>MRGSHHHHHHGSMSNFVNLDIFSNYQKYIDNEQEVRENIRIVVREIEHLSKEAQIKLQIIHSDLSQISAACGLARKQVELCAQKYQKLAELVPAGQYYRYSDHWTFITQRLIFIIALVIYLEAGFLVTRETVAEMLGLK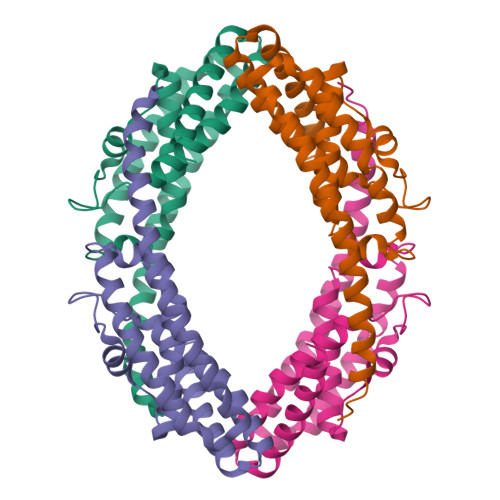ISQSEGFHLDVEDYLLGILQLASELSRFATNSVTMGDYERSLNISHFIGDLNTGFRLLNLKNDGLRKRFDALKYDVKKIEEVVYDVSIRGLSSKEKDQQEEPAVPATE[4x]> RTLRSITSPLVAHRLKPIRQKTKKAVVSILDSEEVCVELVKEYASQEYVKEVLQISSDGNTITIYYPNGGRGFPLADRPPSPTDNISRYSFDNLPEKYWRKYQYASRFVQLVRSKSPKITYFTRYAKCILMENSPGADFEVWFYDGVKIHKTEDFIQVIEKT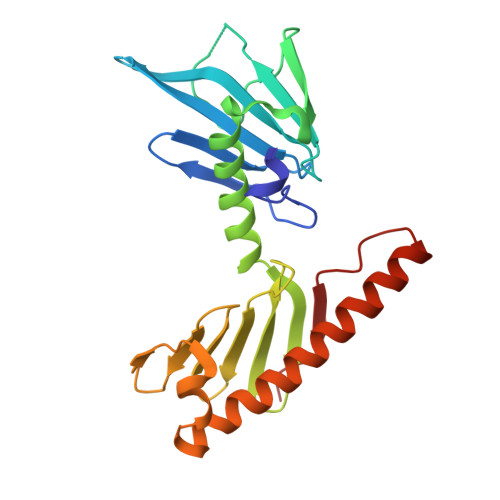GKSYTLKSESEVNSLKEEIKMYMDHANEGHRICLALESIISEEERKTRSAPFFPIIIGRKP> MGHHHHHHMSPNLPGQTTVQVRVPYRVVGLVVGPKGATIKRIQQQTHTYIVTPSRDKEPVFEVTGMPENVDRAREEIEMHIA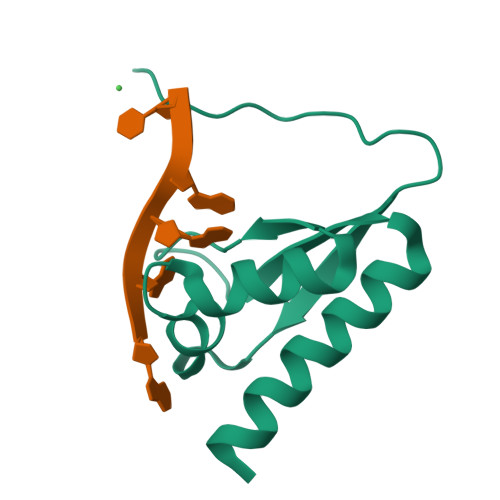MRTG>[2x]MQTKERYQLQRLTLLALLTAMCVVLRIFKIIDIPNVQPVTDIIMLTTLELGAGTGILLAILVMVISNIFLGFGIWTLPQIFAYAACALTVALFARLLPLKSRKFFWLQELLAGFLGLEYGFFVSLGMAGWGGWAAFIAYWVSGLTFDLYHAAGNLAFYPIFYLPLVLGLDRFKKKAGWKQNA;>[2x]MHHHHHHHHHHGENLYFQGSDNIISFDHVTFTYPDSPRPALSDLSFAIERGSWTALIGHNGSGKSTVSKLINGLLAPDDLDKSSITVDGVKLGADTVWEVREKVGIVFQNPDNQFVGATVSDDVAFGLENRAVPRPEMLKIVAQAVADVGMADYADSEPSNLSGGQKQRVAIAGILAVKPQVIILDESTSMLDPEGKEQILDLVRKIKEDNNLTVISITHDLEEAAGADQVLVLDDGQLLDQGKPEEIFPKVEMLKRIGLDIPFVYRLKQLLKERGIVLPDEIDDDEKLVQSLWQLNSKM;>[2x]MAIKFENVSYVYSPGSPLEAIGLDQLNFSLEEGKFIALVGHTGSGKSTLMQHFNALLKPTSGKIEIAGYTITPETGNKGLKDLRRKVSLAFQFSEAQLFENTVLKDVEYGPRNFGFSEDEAREAALKWLKKVGLKDDLIEHSPFDLSGGQMRRVALAGVLAYEPEIICLDEPAAGLDPMGRLEMMQLFKDYQAAGHTVILVTHNMDDVADYADDVLALEHGRLIKHASPKEVFKDSEWLQKHHLAEPRSARFAAKLEAAGLKLPGQPLTMPELADAIKQSLKGGEHE;>[2x]MSKIIIGRYLPGTTFVYRVDPRAKLLTTFYFIIMIFLANNWVSYLVISIFGLAYVFATGLKARVFWDGVKPMIWMIVFTSLLQTFFMAGGKVYWHWWIFTLSSEGLINGLYVFIRFAMIILVSTVMTVTTKPLEIADAMEWMLTPLKLFKVNVGMISLVISIALRFVPTLFDQTVKIMNAQRSRGADFNDGGLVKRAKSVVPMLVPLFIDSLEVALDLSTAMESRGYKGSEGRTRYRILEWSKVDLIPVAYCLLLTILMITTRKH

ECF-transporters are multi-subunit membrane complexes that consist of two ATPases, similar to the ATPases of ABC transporters, and two membrane embedded proteins, not related to any other protein family. The two ATPases and one of the transmembrane proteins, EcfT, form the ‘energizing unit’ or ’ ECF-module’. The other membrane protein, termed S-component, acts as the substrate-binding protein and dynamically associates with the ECF-module to allow for substrate translocation. We demonstrate that ECF-CbrT is a Cbl transporter that catalyses ATP-dependent uptake of Cbl and its precursor Cbi.

We crystallized the ECF-CbrT complex in detergent (n-Dodecyl-β-D-maltopyranoside, DDM) solution and solved a crystal structure to 3.4 Å resolution using molecular replacement with the structure of the folate transporter, ECF-FolT2, from L. delbrueckii as a search model. There are two copies of ECF-CbrT in the asymmetric unit, corresponding to molecules A and B, each of them comprising CbrT, EcfT, EcfA and EcfA’. In both complexes, the two nucleotide-binding domains (NBDs; EcfA and EcfA’) are in a nucleotide-free state, adopting an open conformation with two incomplete ATP-binding sites. CbrT is in a ‘toppled’ orientation in the ECF-CbrT complex with TMs 1, 2, 3 and 4 oriented almost parallel to the membrane plane. Although OH-Cbl was added in excess to the crystallization condition, the substrate was not bound. The apo-state of the toppled S-component was observed before in other ECF-type transporters and likely represents the inward-facing state after substrate release. We hypothesize that the binding site for Cbl is located in a large cavity observed in the CbrT structure. In contrast to ECF-FolT2, and structurally characterized ECF complexes from other organisms, the binding cavity in ECF-CbrT is largely occluded, and not accessible from the cytosol. The occlusion is caused mainly by the position of loop 3, which obstructs access to the cavity in CbrT. We speculate that occlusion of the empty binding site after cytoplasmic release of the substrate may be required for the subsequent reorientation of the S-component, upon release from the ECF module.>AMYSTNAYAELAGPPKIFCKSVSKDPDFRLKQIDYVIPVQQDRSICMNNPLLDISDGFFTYIHYEGINSCKKSDSFKVLLSHGEIVDRGDYRPSLYLLSSHYHPYSMQVINCVPVTCNQSSFVFCHISNNTKTLDNSDYSSDEYYITYFNGIDRPKTKKIPINNMTADNRYIHFTFSGGGGVCLGEEFIIPVTTVINTDVFTHDYCESFNCSVQTGKSLKEICSESLRSPTNSSRYNLNGIMIISQNNMTDFKIQLNGITYNKLSFGSPGRLSKTLGQVLYYQSSMSWDTYLKAGFVEKWKPFTPNWMNNTVISRPNQGNCPRYHKCP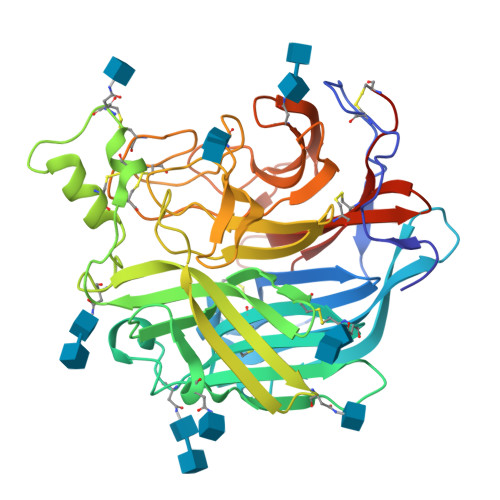EICYGGTYNDIAPLDLGKDMYVSVILDSDQLAENPEITVFNSTTILYKERVSKDELNTRSTTTSCFLFLDEPWCISVLETNRFNGKSIRPEIYSYKIPKYC[2x]>[12x]MAWNQPGNNGQDRDPWGSSKPGGNSEGNGNKGGRDQGPPDLDDIFRKLSKKLGGLGGGKGTGSGGGSSSQGPRPQLGGRVVTIAAAAIVIIWAASGFYTIKEAERGVVTRFGKFSHLVEPGLNWKPTFIDEVKPVNVEAVRELAASGVMLTSDENVVRVEMNVQYRVTNPEKYLYSVTSPDDSLRQATDSALRGVIGKYTMDRILTEGRTVIRSDTQRELEETIRPYDMGITLLDVNFQAARPPEEVKAAFDDAIAARENEQQYIREA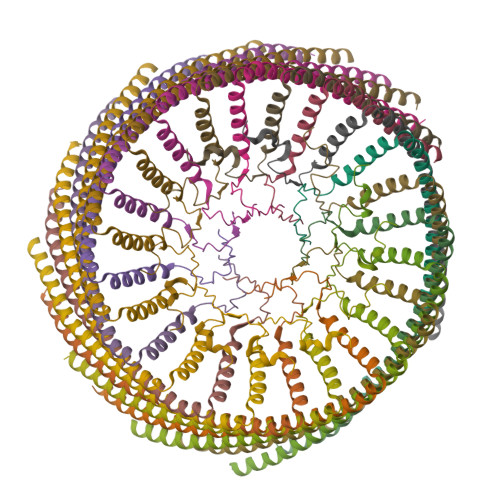EAYTNEVQPRANGQAQRILEEARAYKAQTILEAQGEVARFAKLLPEYKAAPEITRERLYIETMEKVLGNTRKVLVNDKGGNLMVLPLDQMLKGGNAPAAKSDNGASNLLRLPPASSSTTSGASNTSSTSQGDIMDQRRANAQRNDYQRQGE;>MRKSVIAIIIIVLVVLYMSVFVVKEGERGITLRFGKVLRDDDNKPLVYEPGLHFKIPFIETVKMLDARIQTMDNQADRFVTKEKKDLIVDSYIKWRISDFSRYYLATGGGDISQAEVLLKRKFSDRLRSEIGRLDVKDIVTDSRGRLTLEVRDALNSGSAGTEDEVTTPAADNAIAEAAERVTAETKGKVPVINPNSMAALGIEVVDVRIKQINLPTEVSEAIYNRMRAEREAVARRHRSQGQEEAEKLRATADYEVTRTLAEAERQGRIMRGEGDAEAAKLFADAFSKDPDFYAFIRSLRAYENSFSGNQDVMVMSPDSDFFRYMKTPTSATR[12x]> MFFFEFLQ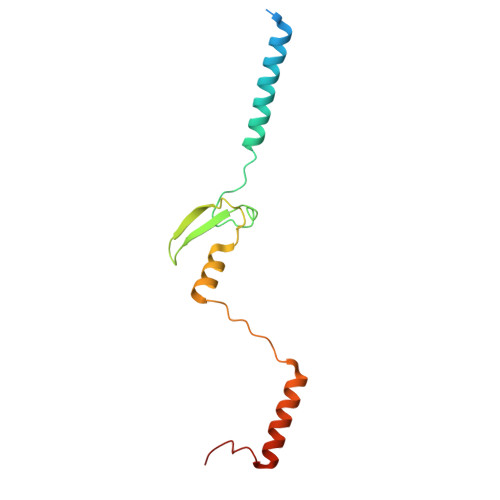GKISDSQKEVDSQAEWYAEYDKLEKARQKRRIWKWRDSDSRDEYAINAEEPVIYIRSSLFGRTEVDPTGKNTNRNHQYLYNLKVLGHKTYTRRDPNELQKAQAEVDTLSAAGRLGPLSPF> GPGSMCTNIVY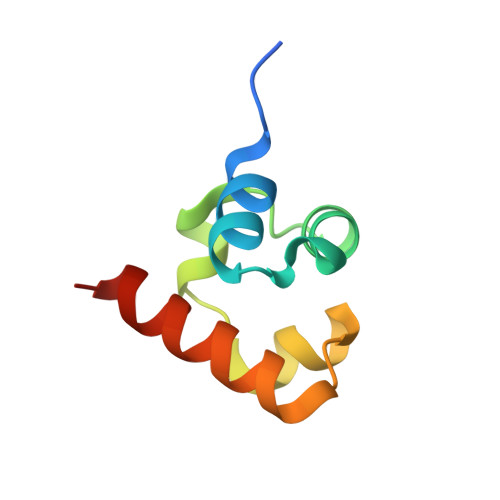EWLKALQLPQYAESFVDNGYDDLEVCKQIGDPDLDAIGVLAPAHRRRILEAVHRLREQD>MHHHHHHSTENLYFQGSSTSCNPSDMSHGYVTVKPRVRLHFVELGSGPAVCLCHGFPESWYSWRYQIPALAQAGYRVLAMDMKGYGESSAPPEIEEYCMEVLCKEMVTFLDKLGLSQAVFIGHDWGGMLVWYMALFYPERVRAVASLNTPFIPANPNMSPLESIKANPVFDYQLYFQEPGVAEAELEQNLSRTFKSLFRASDESVLSMHKVCEAGGLFVNSPEEPSLSRMVTEEEIQFYVQQFKKSGFRGPLNWYRNMERNWKWACKSLGRKILIPALMVTAEKDFVLVPQMSQHMEDWIPHLKRGHIEDCGHWTQMDKPTEV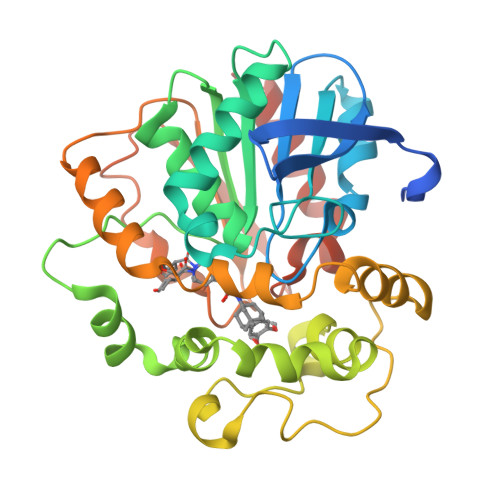NQILIKWLDSDARNPPVVSKM[2x]N-[(1S)-1-benzyl-2-[2-[5-chloro-2-(tetrazol-1-yl)phenyl]ethylamino]-2-oxo-ethyl]-4-hydroxy-2-oxo-1H-quinoline-6-carboxamide | C28 H24 Cl N7 O4 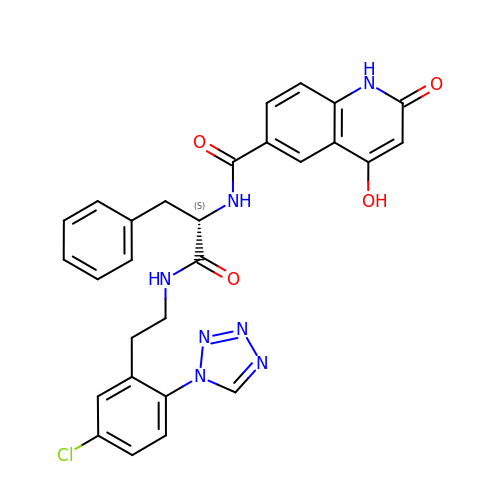| JAUUPTJHJIUVMZ-QHCPKHFHSA-N ACARBOSE DERIVED PENTASACCHARIDE | C31 H53 N O23 | 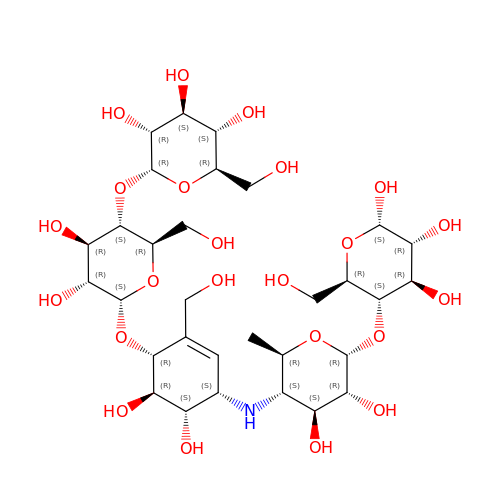JUCZMZWYUIRMPL-NPPSNIQKSA-N> MAMRQCAIYGKGGIGKSTTTQNLVAALAEMGKKVMIVGCDPKADSTRLILHSKAQNTIMEMAAEAGTVEDLELEDVLKAGYGGVKCV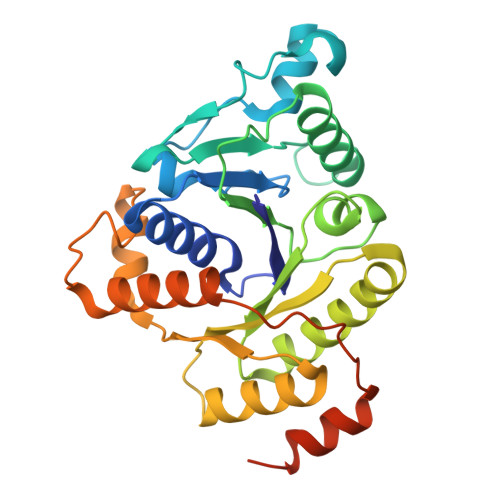ESGGPEPGVGCAGRGVITAINFLEEEGAYEDDLDFVFYDVLGDVVCGGFAMPIRENKAQEIYIVCSGEMMAMYAANNISKGIVKYANSGSVRLGGLICNSRNTDREDELIIALANKLGTQMIHFVPRDNVVQRAEIRRMTVIEYDPKAKQADEYRALARKVVDNKLLVIPNPITMDELEELLMEFGIMEVEDESIVGKTAEEV> GAMEDPVEYPADYFRKSKEIPLYINTTKSLSDLRGYVYQGLKSGNVSIIHVNSYLYGALKDIRGKLDKDWSSFGINIGKAGDTIGIFDLVSLKALDGVLPDGVSDASRTSADDKWLPLYLLGLYRVGRTQMPEYRKKLMDGLTNQCKMINEQFEPLVPEGRDIFDVWGNDSNYTKIVAAVDMFFHMFKKHECASFRYGTIVSRFKDCAALATFGHLCKITGMSTEDVTTWILNREVADEMVQMMLPGQEIDKADSYMPYLIDFGLSSKSPYSSVKNPAFHFWGQLTALLLRSTRARNARQPDDIEYTSLTTAGLLYAYAVGSSADLAQQFCVGDNKY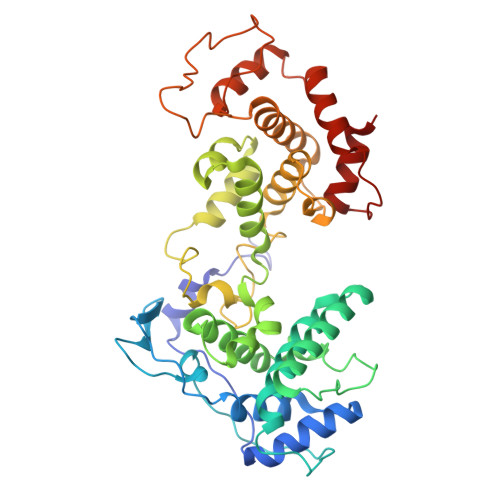TPDDSTGGLTTNAPPQGRDVVEWLGWFEDQNRKPTPDMMQYAKRAVMSLQGLREKTIGKYAKSEFDK>[2x]KAFPVLGIDYTHVRTPFEISLWILLACLMKIGFHVIPTISSIVPESCLLIVVGLLVGGLIKGVGETPPFLQSDVFFLFLLPPIILDAGYFLPLRQFTENLGTILIFAVVGTLWNAFFLGGLMYAVCLVGGEQINNIGLLDNLLFGSIISAVDPVAVLAVFEEIHINELLHILVFGESLLNDAVTVVLYHLFEEFANYEHVGIVDIFLGFLSFFVVALGGVLVGVVYGVIAAFTSRFTSHIRVIEPLFVFLYSYMAYLSAELFHLSGIMALIASGVVMRPYVEANISHKSHTTIKYFLKMWSSVSETLIFIFLGVSTVAGSHHWNWTFVISTLLFCLIARVLGVLGLTWFINKFRIVKLTPKDQFIIAYGGLRGAIAFSLGYLLDKKHFPMCDLFLTAIITVIFFTVFVQGMTIRPLVDLL

Sodium/proton exchanger 1 (NHE1) is an electroneutral secondary active transporter present on the plasma membrane of most mammalian cells and plays critical roles in regulating intracellular pH and volume homeostasis. Calcineurin B-homologous protein 1 (CHP1) is an obligate binding partner that promotes NHE1 biosynthetic maturation, cell surface expression and pH-sensitivity. We find that NHE1 assembles as a symmetrical homodimer, with each subunit undergoing an elevator-like conformational change during cation exchange. Each monomer is made up of a dimerization domain (TMs 1−3 and 7−10) and a core domain (TMs 4−6 and 11−13).

To identify the Na+ binding site, we first prepared the sample in the presence of 150 mM NaCl at pH 7.5, and the corresponding complex structure is termed as NHE1-CHP1Na/7.5. One of the four classes featuring clearly resolved transmembrane helices was selected for focused 3D reconstructions of the transmembrane domain (TMD) of NHE1 and yielded an EM map of 3.3-Å resolution, which is rich in features, including densities for sidechains and associated lipid molecules, allowing us to build a de novo model of the NHE1 dimer. However, we were unable to resolve the CHP1 molecules from this small set of particles, probably due to severe conformational heterogeneity. Superposition of the complex structures determined under different conditions demonstrates that the NHE1 dimer structures are nearly identical in the presence of Na+ ions, at either pH 7.5 or pH 6.5, with a root-mean-square deviation (RMSD) of 0.6 Å for 840 Cα-atom pairs. A large funnel between the dimerization domain and the core domain in each protomer is accessible only from the intracellular side, indicating that in both pH conditions the NHE1-CHP1 complex adopts an inward-facing conformation. A cluster of proton-titratable residues are located inside of the funnel chamber, including E131 in TM2 (E131TM2), D172TM3, D238TM5, D267TM6, and E391TM10, resulting in a highly negatively charged cavity which is suitable for both cation binding and proton sensing. Nevertheless, we did not observe a bound ion in the NHE1-CHP1 complex, possibly due to the moderate resolution of the EM maps. Upon the structural superposition, it is apparent that the cation binding site of PaNhaP is conserved in NHE1. A putative substrate ion is likely to be directly ligated in NHE1 by five oxygen atoms from sidechains of S263TM6, D267TM6, mainchain of V237TM5, and a water molecule. In the context of inward-facing NHE1-CHP1Na/7.5 and NHE1-CHP1Na/6.5 complexes, the CHP1 molecule exhibits high mobility relative to the NHE1 dimer, resulting in featureless CHP1 density in the EM maps.2-chloropyridine-4-carboxylic acid 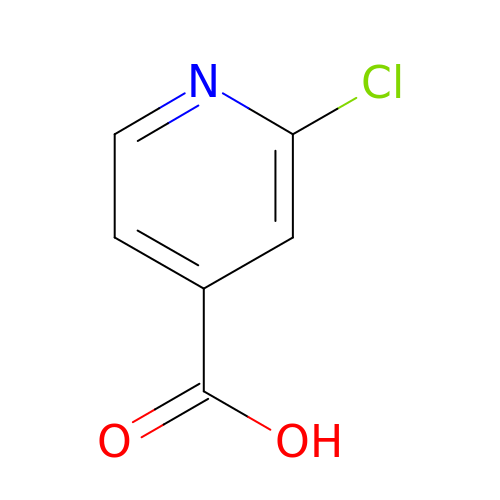| C6 H4 Cl N O2 | QXCOHSRHFCHCHN-UHFFFAOYSA-N>[3x]AAYSQGGGKKKVCYYYDGDIGNYYYGQGHPMKPHRIRMTHNLLLNYGLYRKMEIYRPHK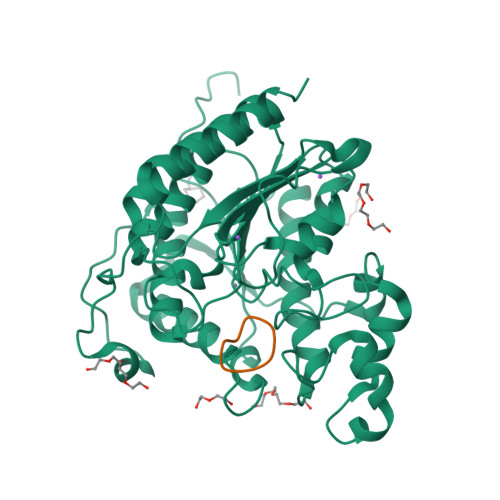ATAEEMTKYHSDEYIKFLRSIRPDNMSEYSKQMQRFNVGEDCPVFDGLFEFCQLSTGGSVAGAVKLNRQQTDMAVNWAGGLHHAKKSEASGFCYVNDIVLAILELLKYHQRVLYIDIDIHHGDGVEEAFYTTDRVMTVSFHKYGEYFPGTGDLRDIGAGKGKYYAVNFPMRDGIDDESYGQIFKPIISKVMEMYQPSAVVLQCGADSLSGDRLGCFNLTVKGHAKCVEVVKTFNLPLLMLGGGGYTIRNVARCWTYETAVALDCEIPNELPYNDYFEYFGPDFKLHISPSNMTNQNTPEYMEKIKQRLFENLRMLPHAPGVQMQAI;>[3x]XNPKQKWG> MSDTMVVNGSGGVPAFLFSGSTLSSYRPNFEANSITIALPHYVDLPGRSNFKLMYIMGFPIDTEMEKDSEYSNKI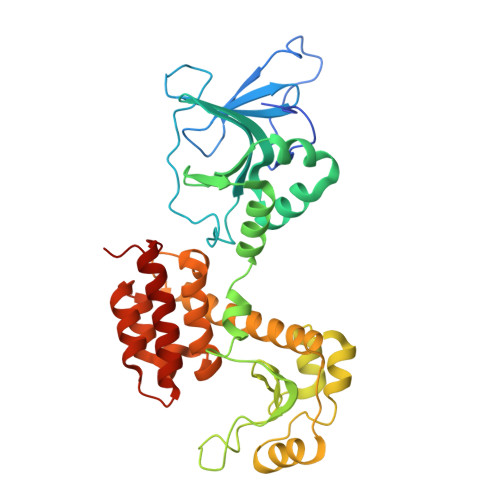RQESKISKTEGTVSYEQKITVETGQEKDGVKVYRVMVLEGTIAESIEHLDKKENEDILNNNRNRIVLADNTVINFDNISQLKEFLRRSVNIVDHDIFSSNGFEGFNPTSHFPSNPSSDYFNSTGVAFGSGVDLGQRSKQDLLNDGVPQYIADRLDGYYMLRGKEAYDKVRTAPLTLSDNEAHLLSNIYIDKFSHKIEGLFNDANIGLRFSDLPLRTRTALVSIGYQKGFKLSRTAPTVWNKVIAKDWNGLVNAFNNIVDGMSDRRKREGALVQKDIDSGLLKLH;> MSDTMVVNGSGGVPAFLFSGSTLSSYRPNFEANSITIALPHYVDLPGRSNFKLMYIMGFPIDTEMEKDSEYSNKIRQESKISKTEGTVSYEQKITVETGQEKDGVKVYRVMVLEGTIAESIEHLDKKENEDILNNNRNRIVLADNTVINFDNISQLKEFLRRSVNIVDHDIFSSNGFEGFNPTSHFPSNPSSDYFNSTGVAFGSGVDLGQRSKQDLLNDGVPQYIADRLDGYYMLRGKEAYDKVRTAPLTLSDNEAHLLSNIYIDKFSHKIEGLFNDANIGLRFSDLPLRTRTALVSIGYQKGFKLSRTAPTVWNKVIAKDWNGLVNAFNNIVDGMSDRRKREGALVQKDIDSGLLKLE> MCSSINEGPYNSPTFGKSLSLKVDGGFNAVSINPSGRDIVLASRQGLYIIDLDDPFTPPRWLHHITPWQVADVQWSPHPAKPYWIVSTSNQKAIIWNLAKSSSNAIEFVLHGHSRAITDINFNPQHPDVLATCSVDTYVHAWDMRSPHRPFYSTSSWRSAASQVKWNYKDPNVLASSHGNDIFVWDLRKGSTPLCSLKGHVSSVNSIDFNRFKYSEIMSSSNDGTVKFWDYSKSTTESKRTVTTNFPIWRGRYLPFGEGYCIMPMVGGNNAVYLINLCDDDDSEQNKKTKLQPIYAFKGHSDRVIDFLWRSRHTCDGDYDDREFQLVTWSKDCDLKLWPISDSIYGKVNFDRGKRLEEKLPDYDYCSYNKEPENRENVQKNEFRRLRENFVTTSGLKKNKTNHITWLSGIRMNSATSQEDLFNETKIQNLGEEVSAIGHKFPKVVFEKISVSTRELCLTLNGPWSEENPDDYIFLRISINFPLNYPNKGDPPKFTIEENSNLTMSKRQEILSNLATIGQKYTDSNLYCLEPCIRFVLGEKVSLEDIEEGQEPLLNFDIADHI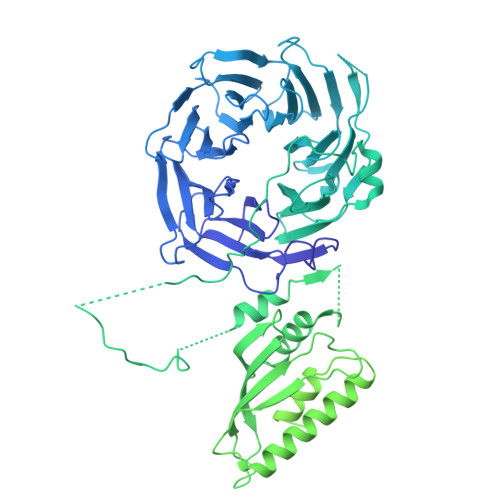DFEELSSLDSSYSDSQNPENLSSQSDIESYKEALVFPDTSNQGLDFGRNLALDTTPVPNGCGSCWTATGELFCFFANEKKPEKKQNAIIKLSQKEAGVEKHPFKIEPQVLYDKEVDSSVITAADELKARPKRYVDTLGLGGGTNGDSRTYFDDETSSDDSFDSVADDWDDILRNDIIVRTKIPILRGNFKAFSSVHSESGKTVESTKKNKNLVISKNFSSLLSDRKELALEYLFMDATPEGFARNNALVAEKFDLDEISHCWQILSDMLIDQSDYDPYTTIWNNHPMGIKWFIKEAIVYFERQQNLQMLAMLCCVILSARRKKIPARYYGQELENMEGTIVFNDNESQNTSFWKGSDAFSTRSRSSTVTPNFYGNHLRGKNIHGGDNSSIRSDDHHARLRTHNTLNGSSKFTEPAQKQGSRAISSSPFHSRMPDIKVELLHDDIIEAYEQEDLLHLEVSDIPKFQTYIYQYSKLLFRWGLPLERVKILKVSTDFRSSYSSQGIPPNNNKKSPYNGVLTHWIENNEFGEEKFLARNCNYCDLRVTRSSFICGNCQHVLHSSCARIWWEIGDECPSGCGCNCPEMFDA The higBA2 TA system from Vibrio cholerae consists of an mRNAse toxin HigB2 and its antitoxin inhibitor HigA2. Antitoxin HigA2 forms a tight complex with HigB2 through its N-terminal disordered region (IDR), which folds upon binding. Here we show that in addition to the primary function of HigA2 IDR to act as a toxin inhibitor, the IDR also contributes to specific and high-affinity recognition of the higBA2 operator to regulate its transcription. The HigA2 folded domain confers specificity towards a single inverted repeat operator sequence, while the IDR enhances its affinity.

To understand the operator specificity of HigA2, its structure in complex with a 17 bp blunt end operator fragment was determined by X-ray crystallography. In the structure with the operator, HigA2 binds to the DNA also as a dimer and induces a 33° bend in the DNA molecule. Only the globular C-terminal HigA2 domain, corresponding to the residues 37-104, could be observed; the N-terminal IDR remains disordered and lacks electron density. HigA2 belongs to the HTH-XRE family of DNA binding proteins and binds each half-site of the operator through its HTH motif formed by helices α2 and α3, while helices α4 and α5 form the HigA2 dimerization interface. Specific base recognition is mediated by four amino acid residues of the recognition helix α3: Arg68, Glu71, Asn72, and Arg77, with the latter adopting a double conformation. These residues interact with both strands of the half-palindrome. In its first conformation, the side chain of Arg77 forms a hydrogen bond with O6 atoms of the guanine 5 and guanine 12 on the opposing DNA strands. In its alternative conformation, the side chain of Arg77 interacts with the phosphate backbone. The side chain of Glu71 forms a hydrogen bond to N6 of the adenine 3 on strand 1, while Arg68 and Asn72 contact N7 atoms of the guanines 14 and 12 on strand 2. In addition to structural changes of the DNA molecule, HigA2 slightly contracts upon DNA binding.

>SNRDLFAELSSALVEAKQHSEGKLTLKTHHVNDVGELNISPDEIVSIREQFNMSRGVFARLLHTSSRTLENWEQGRSVPNGQAVTLLKLVQRHPETLSHIAEL[2x]>GMVRISIAGGNEIDPGSMGLTLFHEHLRLITEVVRWNWPHLYNEDEELKRAIDAVNAAKKYGVKTIIDLTVAGIGCDVRFNEKVAKATGVNIIMGTGFYTYTEIPFYFKNRGIDSLVDAFVHDITIGIQGTNTRAAFVKAVI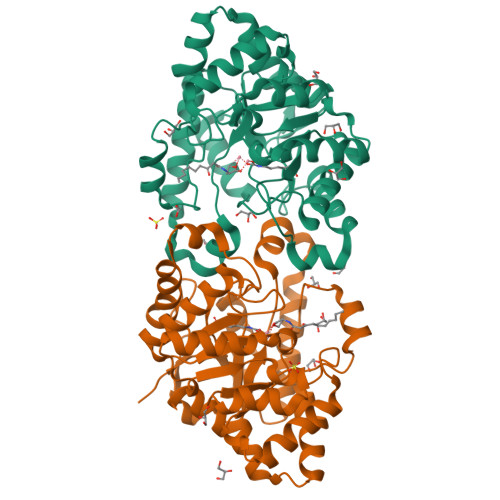DSSGLTKDVEMAIRAAAKAHIKTDVPIITHSFVGNKSSLDLIRIFKEEGVDLARTVIGHVGDTDDISFIEQILREGAFIGLDRFGLDIYLPLDKRVKTAIELIKRGWIDQLLLSHDYCPTIDWYPPEVVRSTVPDWTMTLIFEKVIPRMRSEGITEEQINRVLIDNPRRLFTGR[2x]> QDEISQDKWELARANNYLGLNLLKQLPSNDKTNVFFSPFSVSTAMGMAYAGARGDTLEQLTLNFGYAADELNEGKVLALFKEQLQSTNDLPHDYTLNIANAAVAQEGYGILPEYTDALTSSFGAEYIEADFQKRGQEAIQKINAWVSNRTHGKVQSLFDEPPDFSTRLILLNAIYYKGTWLYEFDKTKTKPRSFYNGGVEKVQVPMMRLKSTLNHTYNAILNADLVDLPYVGNDFSMTIILPREKTGLASLKSVLTSQTLNLALQNMYPKDMKLKLPKFKLDTKYTLKPTLEAMGITKIFSADADLSGISGSRNLYVSDVLHKAVLEVNEEGSEAAAVTGFVIQLRTAAFVTPPPLPKVYVDHPFIFLIRNSKTNTIMFLGEINAL

Here we present the functional and structural characterization of Iripin-8, a salivary serpin from the tick Ixodes ricinus, a European vector of tick-borne encephalitis and Lyme disease. Iripin-8 inhibited multiple proteases involved in blood coagulation and blocked the intrinsic and common pathways of the coagulation cascade in vitro. Moreover, Iripin-8 inhibited erythrocyte lysis by complement, and Iripin-8 knockdown by RNA interference in tick nymphs delayed the feeding time. Based on its inhibitory activity, mainly of proteases of the coagulation cascade, we suggest that its main role as a salivary protein is in the modulation of host blood coagulation and complement activity, with possible function in regulating the immune response.

Finally, we resolved the crystal structure of Iripin-8 at 1.89 Å resolution to reveal an unusually long and rigid reactive center loop that is conserved in several tick species. The crystallographic asymmetric unit contained a single molecule of native Iripin-8. Electron density was of sufficient quality to model all residues from Ser5 to the C-terminus, including the entire RCL. Iripin-8 has the typical native serpin fold with a Cα RMSD (root-mean-square deviation) of 1.93 Å compared with the archetypal serpin alpha-1-antitrypsin (A1AT, 342 of 352 residues). The most remarkable feature of Iripin-8 is its long RCL (11 residues longer on the P′ side), which extends away from the body of the serpin, moving the P1 Arg364 17.8 Å further than the P1 residue of A1AT. This extended conformation is not the result of a crystal contact; rather it forms the basis of a crystal contact with the RCL of a symmetry-related molecule. The P′ extension contains a stretch of proline residues that form a type II polyproline helix, conferring rigidity and extending the P1 residue away from the body of Iripin-8. We can infer from this that the extended RCL is a feature of native Iripin-8 in solution and that it has functional consequences in determining protease specificity and/or inhibitory promiscuity. We also observed several molecules of PEG (polyethylene glycol) originating from the crystallization buffer bound to Iripin-8. One of the binding sites was a deep 109 Å3 cavity in the core structure between helixes A, B, and C.>PWENFDVDGGMDQDIFDINEGLGLDLFEGDIRLDRAQIRNSIIGEKYRWPHTIPYVLEDSLEMNAKGVILNAFERYRLKTCIDFKPWAGETNYISVFKGSGCWSSVGNRRVGKQELSIGANCDRIATVQHEFLHALGFWHEQSRSDRDDYVRIMWDRILSGREHNFNTYSDDISDSLNVPYDYTSVMHYSKTAFQNGTEPTIVTRISDFEDVIGQRMDFSDSDLLKLNQLYNCSSSLSFMDSCSFELENVCGMIQSSGDNADWQRVSQVPRGPESDHSNMGQCQGSGFFMHFDSSSVNVGATAVLESRTLYPKRGFQCLQFYLYNSGSESDQLNIYIREYSADNVDGNLTLVEEIKEIPTGSWQLYHVTLKVTKKFRVVFEGRKGSGASLGGLSIDDINLSETRCPHHIWHIRNFTQFIGSPNGTLYSPPFYSSKGYAFQIYLNLAHVTNAGIYFHLISGANDDQLQWPCPWQQATMTLLDQNPDIRQRMSNQRSITTDPFMTTDNGNYFWDRPSKVGTVALFSNGTQFRRGGGYGTSAFITHE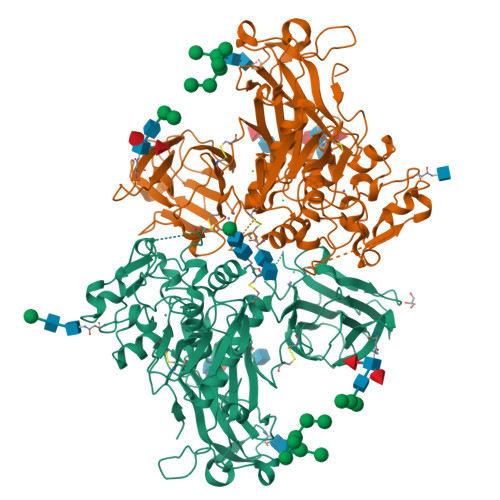RLKSRDFIKGDDVYILLTVEDISHLNSTQIQLTPAPSVQDLCSKTTCK[2x]> MAKREPIHENSTRTEWEGKIAKLNSVDQATKFIQDFRVAYSSP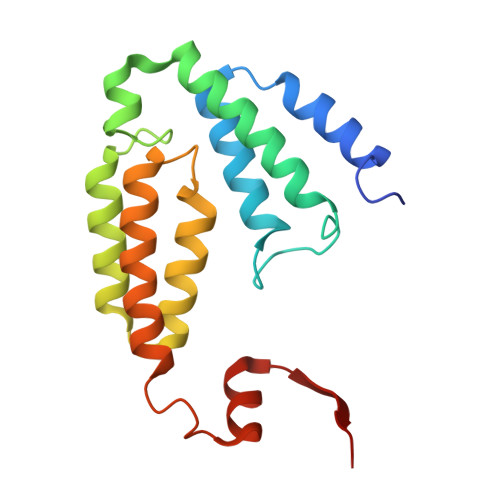FRKSYDLDVDYQYIERKIEERLSVLKTEKLSVADLVTKATTGEDAAAVEAAWIAKMKAAESKYAAERIHIEFRQLYKPPVLPVNVFLRTDAALGTILMELRNTDYYATPLEGLRKERGVKVLHLQA> RSYPAIPRIYAETTLNMLLKRAKKPRVHSIDEYLKDGGYQALEKALNMSPEEIIDWVDKSTLRGRGGAGFPTGKKWKFAVQNPGPRYFICNADESEPGTFKDRIIIERDPHLLIEGIIISSYAIGANEAYIYIRGEYPAGYYILRDAIEEAKKKGFLGKNILGSGFDLEIYVARGAGAYICGEETALIESLEGKRGHPRLKPPYPVQKGLWGKPTVVNNVETIANVPFII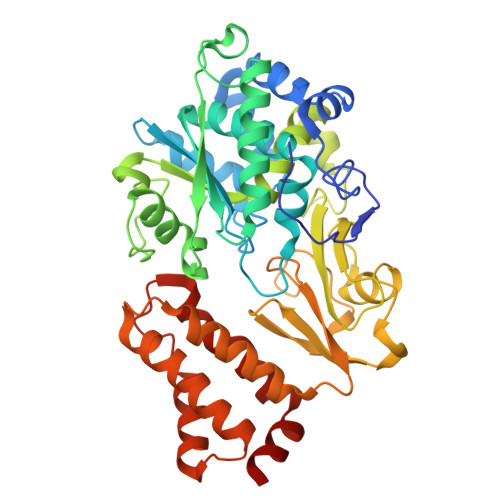SMGWEEYRYIGPSDYAGPKLFPVSGKVKKPGVYELPMNTTLREVIFKYAGGTLGNKKVKAVFSGALDCFSSEELDIPMDYSPLGFGGTGTVIVLTEEDDIVEAALKIAEFYEHETCGQCTPCRVGCYEQANLLEKIYKGEATEQDWEGFDFVNRNIQPTSICGLGAVAGRLIRQTLEKFPEEWEKYRK> MGSSHHHHHHSQDPGWKFSNGKRRPPHKATVTVTDKNGVVKHKSNLVSGNMTEAEKKLGFPNNSLATHTENRATRLIDLNQGDTMLIEGQY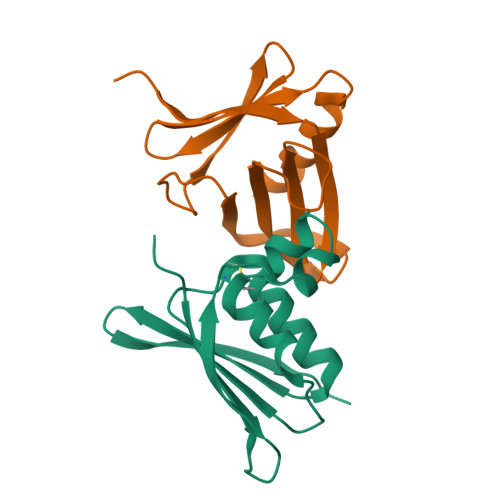RPCPRCKGAMRVKAEESGAKVIYTWPEDGDLKKREWEGTPCDKK;> MTKSKMLSNIVIQEVKFAIEDYCAILSFASDSYEVPEQYFIITRSTTERSGGIPEGDIYLESNLFLDFNPYGLSGYLLSEPNCVDLLIEPNNYVRLRLIEKIDILEVENHLKFLFDN>MTTVIDATMAYRFLEEATDSSSSSSSSKLESSPVDAVLFVGMSLVLGIASRHLLRGTRVPYTVALLVIGIALGSLEYGAKHNLGKIGHGIRIWNEIDPELLLAVFLPALLFESSFSMEVHQIKRCLGQMVLLAVPGVLISTACLGSLVKVTFPYEWDWKTSLLLGGLLSATDPVAVVALLKELGASKKLSTIIEGESLMNDGTAIVVFQLFLKMAMGQNSDWSSIIKFLLKVALGAVGIGLAFGIASVIWLKFIFNDTVIEITLTIAVSYFAYYTAQEWAGASGVLTVMTLGMFYAAFARTAFKGDSQKSLHHFWEMVAYIANTLIFILSGVVIAEGILDSDKIAYQGNSWRFLFLLYVYIQLSRVVVVGVLYPLLCRFGYGLDWKESIILVWSGLRGAVALALSLSVKQSSGNSHISKETGTLFLFFTGGIVFLTLIVNGSTTQFVLRLLRMDILPAPKKRILEYTKYEMLNKALRAFQDLGDDEELGPADWPTVESYISSLKGSEGELVHHPHNGSKIGSLDPKSLKDIRMRFLNGVQATYWEMLDEGRISEVTANILMQSVDEALDQVSTTLCDWRGLKPHVNFPNYYNFLHSKVVPRKLVTYFAVERLESACYISAAFLRAHTIARQQLYDFLGESNIGSIVINESEKEGEEAKKFLEKVRSSFPQVLRVVKTKQVTYSVLNHLLGYIENLEKVGLLEEKEIAHLHDAVQTGLKKLLRNPPIVKLPKLSDMITSHPLSVALPPAFCEPLKHSKKEPMKLRGVTLYKEGSKPTGVWLIFDGIVKWKSKILSNNHSLHPTFSHGSTLGLYEVLTGKPYLCDLITDSMVLCFFIDSEKILSLQSDSTIDDFLWQESALVLLKLLRPQIFESVAMQELRALVSTESSKLTTYVTGESIEIDCNSIGLLLEGFVKPVGIKEELISSPAALSPSNGNQSFHNSSEASGIMRVSFSQQATQYIVETRARAIIFNIGAFGADRTLHRRPSSLTPPRSSSSDQLQRSFRKEHRGLMSWPENIYAKQQQEINKTTLSLSERAMQLSIFGSMVNVYRRSVSFGGIYNNKLQDNLLYKKLPLNPAQGLVSAKSE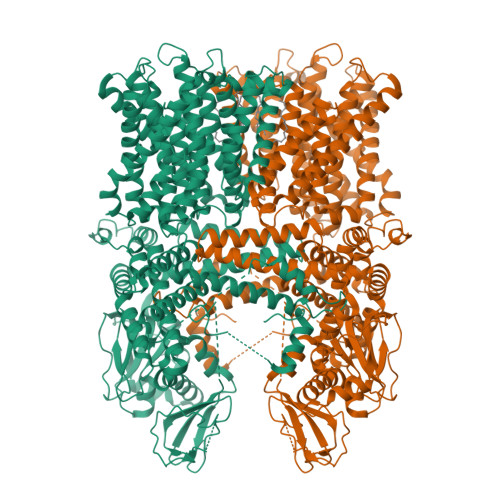SSIVTKKQLETRKHACQLPLKGESSTRQNTMVESSDEEDEDEGIVVRIDSPSKIVFRNDL[2x]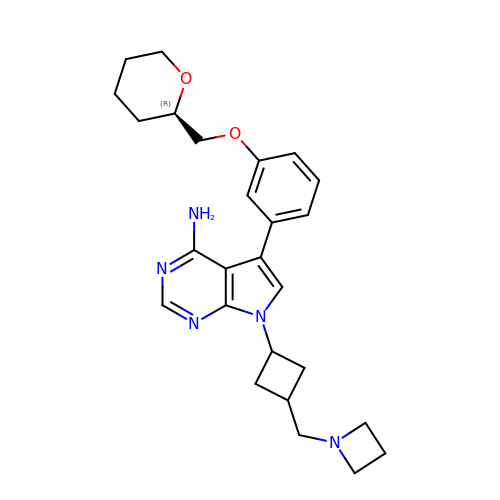7-[3-(azetidin-1-ylmethyl)cyclobutyl]-5-[3-[[(2~{R})-oxan-2-yl]methoxy]phenyl]pyrrolo[2,3-d]pyrimidin-4-amine | C26 H33 N5 O2 | UTHVKVUADCCITP-KAGYGMCKSA-N>MGSSHHHHHHSQDPNSSSARLQVDKLDYDIPTTENLYFQGSMRRSVYLDNTIEFLRGRVYLGAYDYTPEDTDELVFFTVEDAIFYNSFHLDFGPMNIGHLYRFAVIFHEILNDPENANKAVVFYSSASTRQRANAACMLCCYMILVQAWTPHQVLQPLAQVDPPFMPFRDAGYSNADFEITIQDVVYGVWRAKEKGLIDLHSFNLESYEKYEHVEFGDFNVLTPDFIAFASPQEDHPKGYLATKSSHLNQPFKSVLNFFANNNVQLVVRL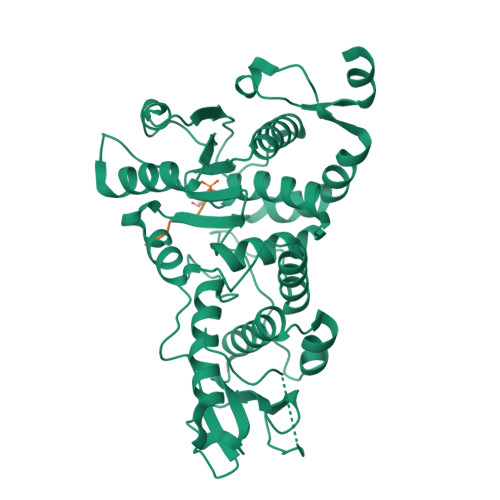NSHLYNKKHFEDIGIQHLDLIFEDGTCPDLSIVKNFVGAAETIIKRGGKIAVHSKAGLGRTGCLIGAHLIYTYGFTANECIGFLRFIRPGMVVGPQQHWLYLHQNDFREWKYTTRISLKPSEAIGGLYPLISLEEYRLQKKKLKD[2x];> HRELGSPLKK> MHHHHHHHHHHSGDEVDAGSGHMTNEEPLPKKVRLSETDFKVMARDELILRWKQYEAYVQALEGKYTDLNSNDVTGLRESEEKLKQQQQESARRENILVMRLATKEQEMQECTTQIQYLKQVQQPSVAQLRSTMVDPAINLFFLKMKGELEQTKDKLEQAQNELSAWKFTPDSQTGKKLMAKCRMLIQENQELGRQLSQGRIAQLEAELALQKKYSEELKSSQDELNDFIIQL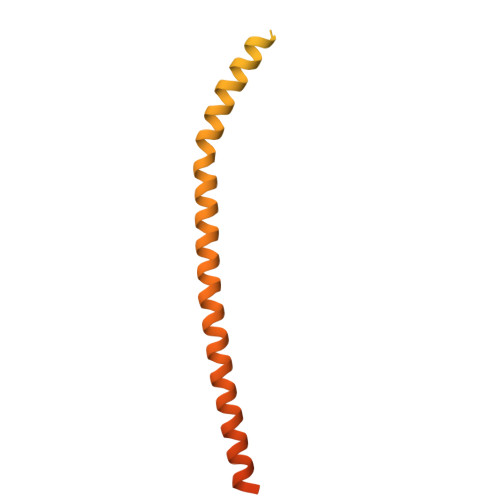DEEVEGMQSTILVLQQQLKETRQQLAQYQQQQSQASAPSTSRTTASEPVEQSEATSKDCSRL5'-O-{(R)-hydroxy[(L-lysylamino)oxy]phosphoryl}adenosine 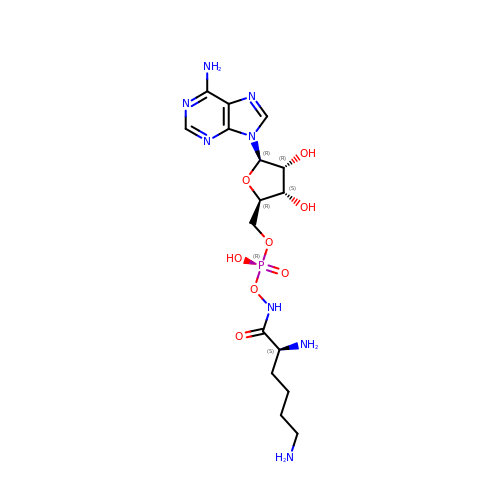| C16 H27 N8 O8 P | UZJSLDPAROCUBS-LEJQEAHTSA-N>APTSSSTKKTQLQLEHLLLDLQMILNGINNYKNPKLTRMLTFKFYMPKKATELKHLQCLEEELKPLEEVL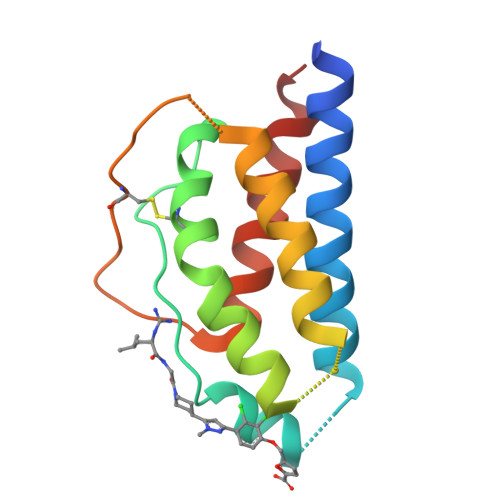NLAQSKNFHLRPRDLISNINVIVLELKGSETTFMCEYADETATIVEFLNRWITFCQSIISTL[4x]> MAFRNTFTTPGKFSTVSKNIVLLLIWRVKVFLRAEGFAHSLVMLPVSLYSKILLCDVKKKIVYFHCCTRKKSMLR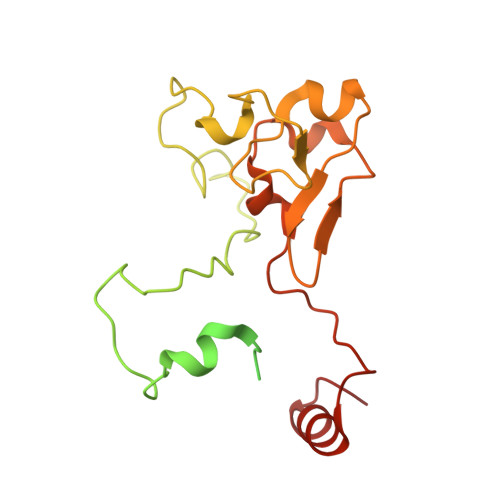RCPCVWPDGPTKSSVSIGTAFTLQKRFLKIAKSAFGFYLARRGQRKYPFLRRPHIKNTHSMNPSAPYFWSFMTAKSQMAFLPEENYITGDWTGKFFVSKRQVYTLQHATSGAKVRVKSFPSIFEFNSPSRWNIGKEMNTLTKPRMDLIDEQMLTKKQRLDYVRAGLLPK> MANFLKNLHPLLRRDRNKKDNQDPNFALIDALNEEMNQVEKDAIESKLQSSLKTSTSEYLDKFGDWFGVYRKTDEKDDVYRARIIKYLLLKRGTNNAIIDAIKDYLGRDDIDVSVYEPFTNIFYTNKSHLNGEDHLMGYYYRFAVINVSIGDYFPVEIIDVINEFKPAGVTLYVTYDGASTIRGGAIIKWLDGLPKIETYQEFDRFTGYDDTFYGHINMNQSKDTDNSSSDI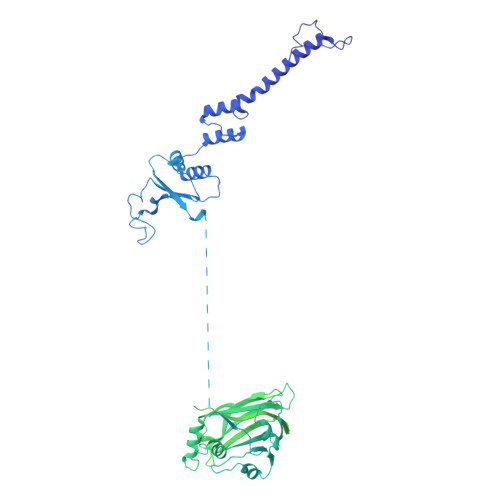FKTNHSLINSLDVLTGSSSVGRQYINYGYVTSYVYNPGMTSSVNQISASTEGRGQEVPTDYYMYTSTKNNNTVELSMQTTSGVSYLYNNFNFRDYMSKYRPQVDLQSDEARRIVSDYIKELSIDYYLSAVIPPDESIEIKLQVYDFSINRWLTVSINNLSFYEKNIGSNIGYIKDYLNSELNMFTRLEINAGKRDSVDIKVNYLDLMFYYYERGIYTIKPYKALIENYLDISRETYVEAFKIASLSNGDIITKTGFQPIGYLKLVGNYENTIPSTINIVAKDTDNNPIESNELDVYNTVENRNLLQSYKGVNTIAREITSTKEFTVSGWAKEIYSTNYLSKVLKPGKVYTLSFDMEITGNDPTLKSYSDNHGIYLYSNTKGIVVNGVKSMERTIGNKVSVTQTFTAPTITDHRLLIYTGRYTSDGKASTPPVFFNTVKITELKLTEGSSKLEYSPAPEDKPNVIEKGIKFNNILTNIQTLSINSDTILKNVTLYYSYYGDSWVELKTLGNISTGETTETNNLIDLYGLQTVDYSNINPMSKVSLRSIWNVKLGELNNQEGSLSNMPNDYFNAVWQDIDKLSDIELGSMRMVKDTEGGVFDGATGEIIKATLFNVGAYTDLDMLAYTLTNYTEPLTLGSSRLISELKEELLTSESFNVDNRIKVIDSIYEELPNTSIIKNGFVEREVTGSKYLDYGLYEPIEDGTRYKLIVEGEFKDNIEFISLYNSNPNFNETFIYPSEIINGVAEKEFIAKPSTEDKPRLNTDVRIYIRPYDSTISKVRRVELRKV>[2x]MRPHRAFSPGLTGVLPLRETRHLVEVLRARVGDRFT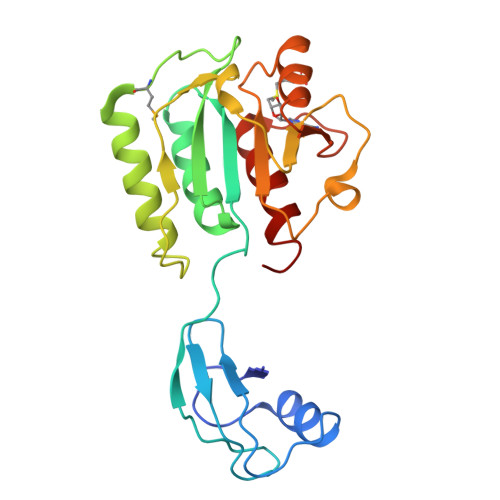VFDGEREALAEVVDLGPPLRYRVLEERRPEREVGVEVVLYVALLKGDKLAEVVRAATELGATRIQPLVTRHSVPKEMGEGKLRRLRAVALEAAKQSGRVVVPEVLPPIPLKAVPQVAQGLVAHVGATARVREVLDPEKPLALAVGPEGGFAEEEVALLEARGFTPVSLGRRILRAETAALALLALCTAGEGR> MSTIEERVKKIIGEQLGVKQEEVTNNASFVEDLGADSLDTV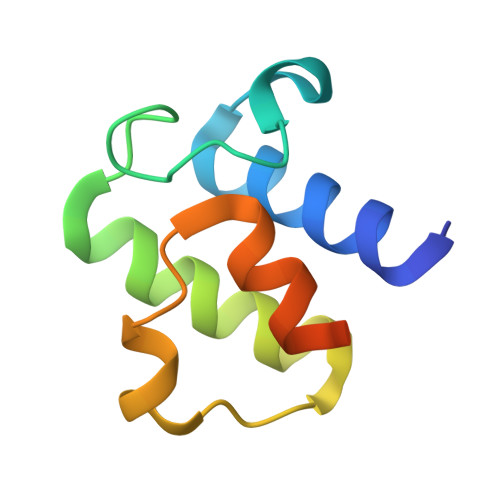ELVMALEEEFDTEIPDEEAEKITTVQAAIDYINGHQASHHHHHH> QDLTVKMTDLQTGKPVGTIELSQNK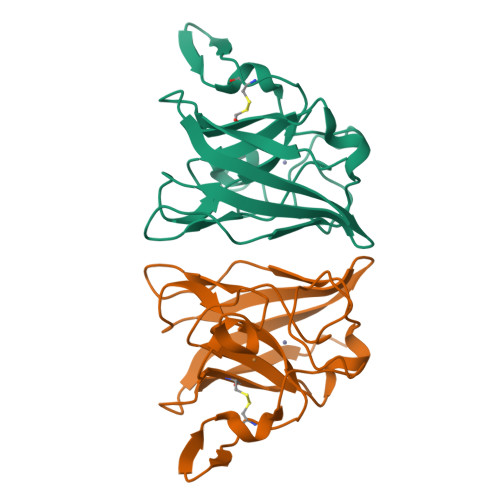YGVAFIPELADLTPGMHGFHIHQNGSCASSEKDGKVVLGGAAGGHYDPEHTNKHGFPWTDDNHKGDLPALFVSANGLATNPVLAPRLTLKELKGHAIMIHAGGDNHSDMPKALGGGGARVACGVIQ>MDSKYQCVKLNDGHFMPVLGFGTYAPAEVPKSKALEAVKLAIEAGFHHIDSAHVYNNEEQVGLAIRSKIADGSVKREDIFYTSKLWSNSHRPELVRPALERSLKNLQLDYVDLYLIHFPVSVKPGEEVIPKDENGKILFDTVDLCATWEAMEKCKDAGLAKSIGVSNFNHRLLE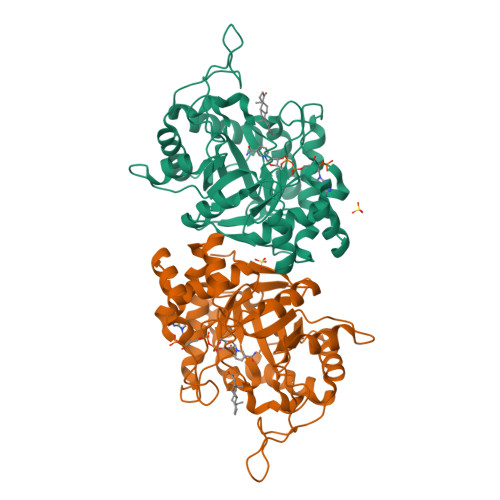MILNKPGLKYKPVCNQVECHPYFNQRKLLDFCKSKDIVLVAYSALGSHREEPWVDPNSPVLLEDPVLCALAKKHKRTPALIALRYQLQRGVVVLAKSYNEQRIRQNVQVFEFQLTSEEMKAIDGLNRNVRYLTLDIFAGPPNYPFSDEY[2x]> QFMQNTEALCDVKGFAPFSKDNGIRIGSRGHVFVIREPFVSCSPTECRTFFLTQGSLLNDKHSNGTEKDRSPYRTLMSVEIGQSPNVYQARF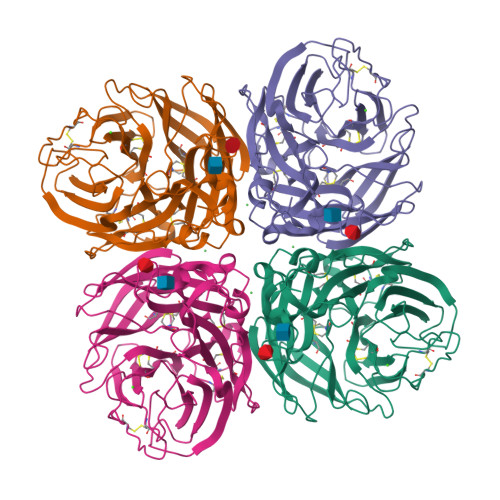EAVAWSATACHDGKKWMTIGVTGPDAKAVAVVHYGGIPTDVINSWAGDILRTQESSCTCILGECYWVMTDGPANRQAQYRAFKAKQGKIIGQVEISFNGGHIEECSCYPNDGKVECVCRDNWTGTNRPVLVISPDLSYRVGYLCAGLSSDTPRGEDSQFTGSCTSPVGNQGYGVKGFGFRQGNDVWMGRTISRTSRSGFEILKVRNGWVQTSKEQIKRQVVVDNLNRSGYSGSFTLPVELTKRDCLVPCFWVEMIRGKPAEKTIWTSSSSIVMCGVDHEVADWSWHDGAILPFDID>SNAMPLPKSLKYGDTIGIYSPSSPVTYTSPKRFERAKSYLLQKGFHILEGSLTGRYDYYRSGSIQERAKELNALIRNP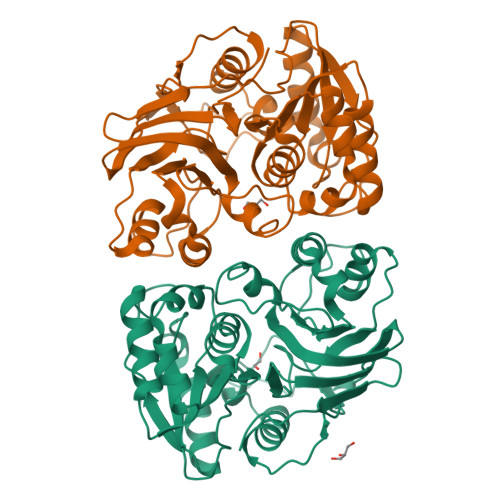NVSCIMSTIGGMNSNSLLPYIDYDAFQNNPKIMIGYADATALLLGIYAKTGIPTFYGPALVPSFGEFEPFVDDTYKYFLETLLHDQALPYNIKQPLFWSDEFINWEEKTKEKELRPNNWISVTNGQATGRVIGGNLNTIQGIWGSPYMPCIQEGDILFIEDSSKDAATIERSFSFLKINGVFDKVSGIILGKHEQFDDCGTNRKPYEILLEVLQNQRIPLLADFDCCATHPMITMPIGVQVKMDATNKTIHILEKWKI[2x]> MASHHHHHHVSAGESVQITLPKNEVQLNAYVLQEPPKGETYTY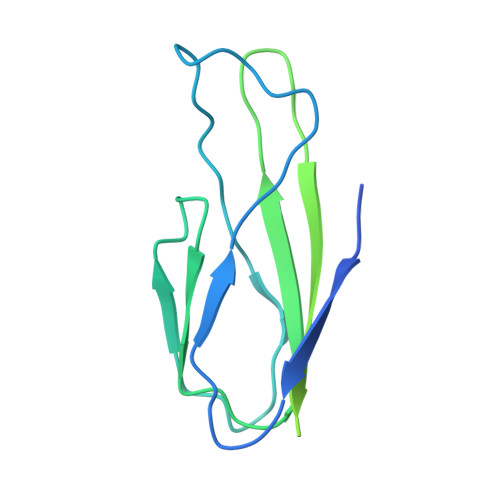DWQLITHPRDYSGEMEGKHSQILKLSKLTPGLYEFKVIVEGQNAHGEGYVNVTVKPEPRKNRPPIAIVSPQFQEISLPTTSTVIDGSQSTDDDKIVQYHWEELKGPLREEKISEDTAILKLSKLVPGNYTFSLTVVDSDGATNSTTANLTVNKAVD> GPLGSPEFDCHLSDMLQQLHSVNASKPSERGLVRQEEAEDPACIPIFWVSKWVDYSDKYGLGYQLCDNSVGVLFNDSTRLILYNDGDSLQYIERDGTESYLTVSSHPNSLMKKITLLKYFRNYMSEHLLKAGANITPREGDELARLPYLRTWFRTRSAIILHLSNGSVQINFFQDHTKLILCPLMAAVTYIDEKRDFRTYRLSLLEEYGCCKELASRLRYARTMVDKLLSSR;> XDPPLHSTAX

The PBD domain is responsible for the proper cellular localization of Plk1 through an array of phosphorylation-dependent protein–protein interactions mediated by the phosphopeptide-binding groove. Disrupting these interactions has shown potential as a strategy for anticancer therapy. The discovery of an auxiliary flexible pocket on the PBD surface, which is involved in binding a peptide derived from polo-box interacting protein 1 (PBIP1), has been recently reported. Our objective was to prepare more potent ligands of the PBD by improving binding to this auxiliary pocket by optimizing the hydrophobic interactions whilst retaining the key hydrogen bond.

To further study the molecular recognition of the pocket, we expanded the series of PBIP1-derived peptides to include non-amino acid N-terminal residues, focusing on, but not limited to, hydrophobic aromatic ring systems. In addition, the two double-ring aromatic systems 3 j,k were tested, both giving high ΔΔTm values indicative of hydrophobic pocket binding. The structures of these compounds suggest that they are able to insert their benzene rings into the pocket, reinforcing the suggestion of its selectivity for aromatic moieties. Peptides identified in the assay as pocket binders have in general shown higher affinity than those not utilizing the pocket, and all the most potent ligands (3 d, 3 f, 3 j, and 3 k, colored purple) also bind to the pocket exhibiting the highest ΔΔTm>4.0 K. None of the peptides designated as weak binders (in blue) showed pocket binding. To confirm the binding modes, we co-crystallized two representative examples with the PBD, the leucine-based peptide 2 a (ΔΔTm=0.3 K) and the most potent ligand 3 j (ΔΔTm=4.1 K). In contrast, 3 j bound in a way similar to 1 a, retaining the key hydrogen bond and the benzene ring of thiophene was inserted into the pocket, mimicking the phenylalanine of 1 a.>MHHHHHHLKFMLATNICIFTIKNKPASVRERFNLNQGKMCISSVTLMELIYGAEKSQMPERNLAVIEGFVSRIDVLDYDAAAATHTGQIRAELARQGRPVGPFDQMIAGHARSRGLIIVTNNTREFERVGGLRTE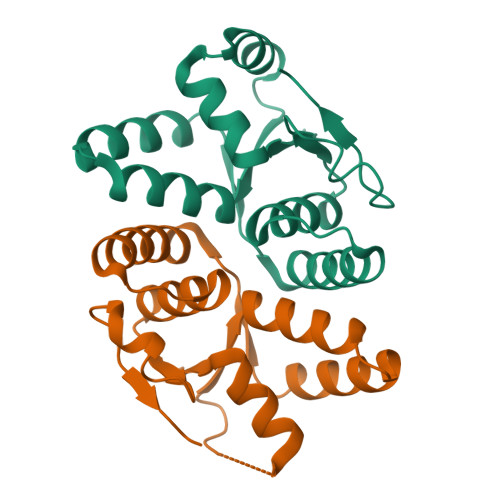DWS[2x]(S)-N-((5-(ethylsulfonyl)pyridin-2-yl)methyl)-7-isopropyl-6-(((1r,4S)-4-(trifluoromethyl)cyclohexyl)methyl)-6,7-dihydro-5H-pyrrolo[3,4-b]pyridine-3-carboxamide 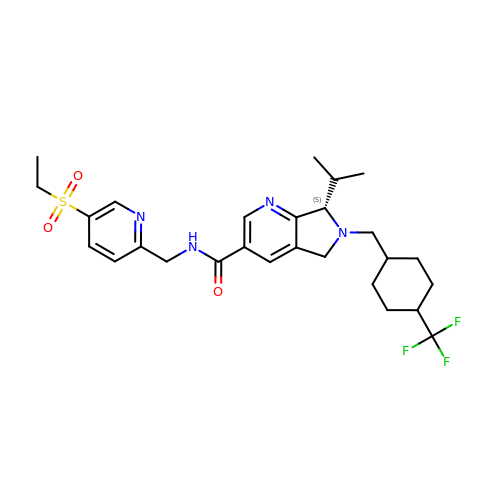| C27 H35 F3 N4 O3 S | XUYMIRYNRKXKOR-HMHJJOSWSA-N>MKEVGSHFDDFVTNLIEKSASLDNGGCALTTFSVLEGEKNNHRAKDLRAPPEQGKIFIARRSLLDELLEVDHIRTIYHMFIALLILFILSTLVVDYIDEGRLVLEFSLLSYAFGKFPTVVWTWWIMFLSTFSVPYFLFQHWATGYSKSSHPLIRSLFHGFLFMIFQIGVLGFGPTYVVLAYTLPPASRFIIIFEQIRFVMKAHSFVRENVPRVLNSAKEKSSTVPIPTVNQYLYFLFAPTLIYRDSYPRNPTVRWGYVAMKFAQVFGCFFYVYYIFERLCAPLFRNIKQEPFSARVLVLCVFNSIL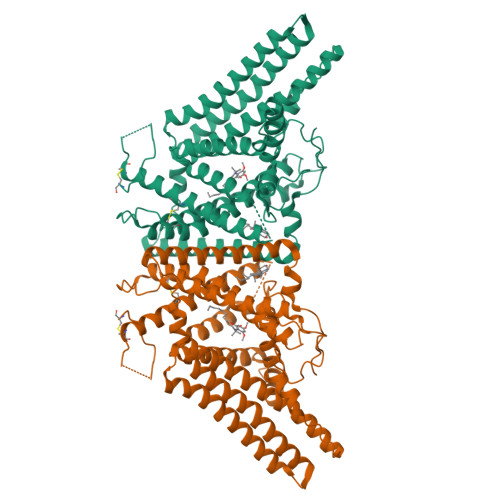PGVLILFLTFFAFLHCWLNAFAEMLRFGDRMFYKDWWNSTSYSNYYRTWNVVVHDWLYYYAYKDFLWFFSKRFKSAAMLAVFAVSAVVHEYALAVCLSFFYPVLFVLFMFFGMAFNFIVNDSRKKPIWNVLMWTSLFLGNGVLLCFYSQEWYARQHCPLKNPTFLDYVRPRSWTCRYVF[2x]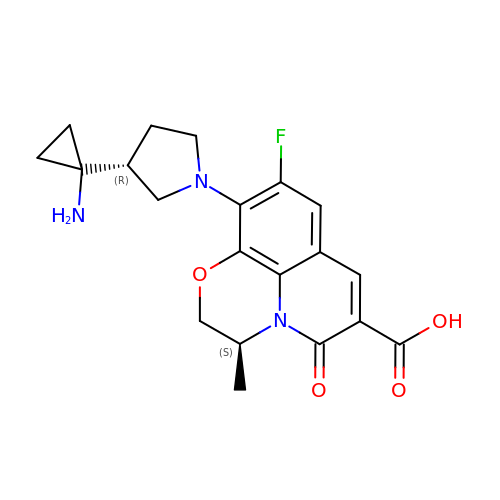(3S)-10-[(3R)-3-(1-aminocyclopropyl)pyrrolidin-1-yl]-9-fluoro-3-methyl-5-oxo-2,3-dihydro-5H-[1,4]oxazino[2,3,4-ij]quinoline-6-carboxylic acid | C20 H22 F N3 O4 | KUJKUYSIFHKKCZ-CMPLNLGQSA-N> AKINQPEYKAANGKWEIIEFPEKYRQNTIHAALLRTGKVLMVAGSGNNQDNSDDKQYDTRIWDPVKGTIKKVPTPSDLFCTGHTQLANGNLLIAGGTKRYEKLKGDVTKAGGLMVVHNENPDKPITLPAGTKFTGKENGKTFVSKDPVLVPRAEKVFDPATGAFVRNDPGLGRIYVEAQKSGSAYETGTEDNYRVQGLSGADARNTYGIAQKLALDKKDFQGIRDAFEFDPVAEKYIKVDPMHEARAYPTLTTLGDGKILSVSGLDDIGQLVPGKNEVYDPKTKAWTYTDKVRQFPTYPALFLMQNGKIFYSGANAGYG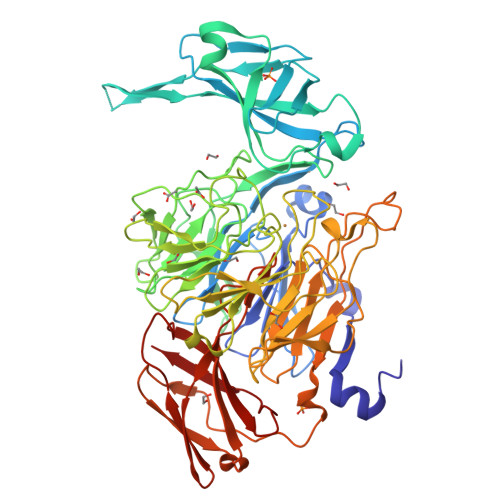PDDVGRTPGVWDVETNKFTKVPGMSDANMLETANTVLLPPAQDEKYMVIGGGGVGESKLSSEKTRIADLKADDPKFVDGPSLEKGTRYPQASILPDDSVLVSGGSQDYRGRGDSNILQARLYHPDTNEFERVADPLVGRNYHSGSILLPDGRLMFFGSDSLYADKANTKPGKFEQRIEIYTPPYLYRDSRPDLSGGPQTIARGGSGTFTSRAASTVKKVRLIRPSASTHVTDVDQRSIALDFKADGDKLTVTVPSGKNLVQSGWYMMFVTDGEGTPSKAEWVRVP> MAVKVEYDLKRLRNIGIAAHIDAGKTTTTERILYYTGRIHKIAEVHEGAATMDFMEQERERGITITAAVTTCFWKDHRINIIDAPGHVDFTIEVERSMRVLDGAIVVFDSSQGVEPQSETVWRQAEKYKVPRIAFANKMDKTGADLWLVIRTMQERLGARPVVMQLPI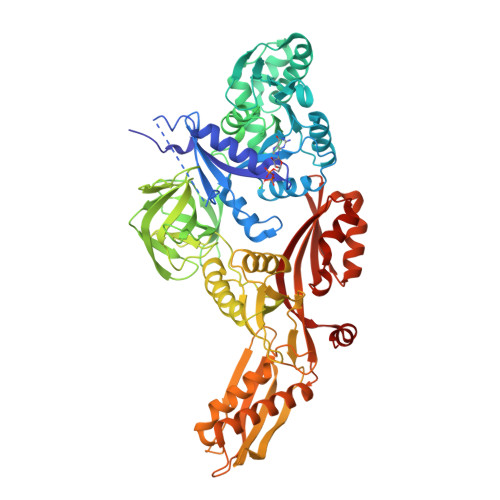GREDTFSGIIDVLRMKAYTYGNDLGTDIREIPIPEEYLDQAREYHEKLVEVAADFDENIMLKYLEGEEPTEEELVAAIRKGTIDLKITPVFLGSALKNKGVQLLLDAVVDYLPSPLDIPPIKGTTPEGEVVEIHPDPNGPLAALAFKIMADPYVGRLTFIRVYSGTLTSGSYVYNTTKGRKERVARLLRMHANHREEVEELKAGDLGAVVGLKETITGDTLVGEDAPRVILESIEVPEPVIDVAIEPKTKADQEKLSQALARLAEEDPTFRVSTHPETGQTIISGMGELHLEIIVDRLKREFKVDANVGKPQVAYRETITKPVDVEGKFIRQTGGRGQYGHVKIKVEPLPRGSGFEFVNAIVGGVIPKEYIPAVQKGIEEAMQSGPLIGFPVVDIKVTLYDGSYHEVDSSEMAFKIAGSMAIKEAVQKGDPVILEPIMRVEVTTPEEYMGDVIGDLNARRGQILGMEPRGNAQVIRAFVPLAEMFGYATDLRSKTQGRGSFVMFFDHYQEVPKQVQEKLIKGQ>[4x]NNMFLVVALDGGREADAVAVMKAAKERGIKIILWLAGDVERLKRLFEKAKELGTDIA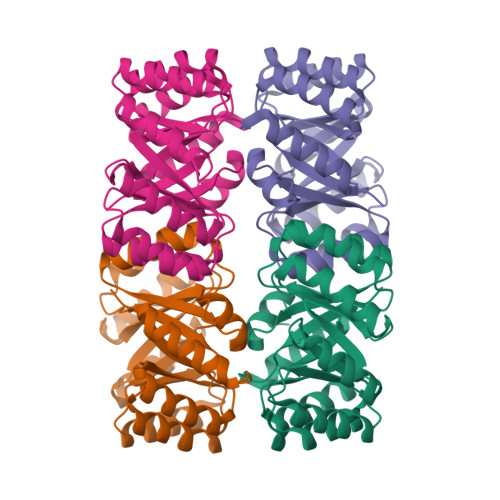GIILDGAPLEKLRPVIKLAAEFGAALFLANMPDAATAEEAIKIAKEEGLEVYLLADLDNLDTVLALAKKYGAKVIAKVDKVEDLKKIVEKVKAHGTDILAGILISPLKPEMVDTLKKAIDELPGVKTVFLSGVSANPALAVEVTKFLLEKGIAVGVLERVPPEEVVALLDAGALEHHHHHH> CGGT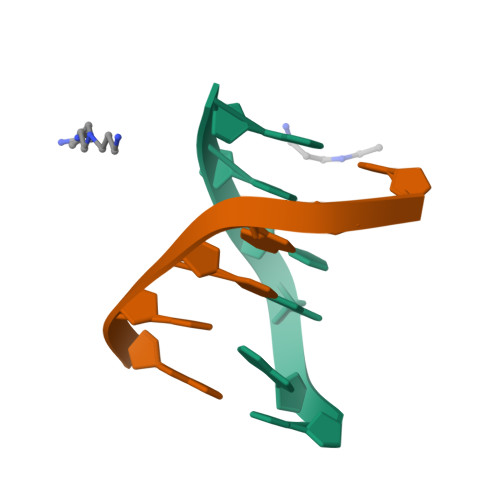GG;> CCACCG>AEYVRALFDFNGNDEEDLP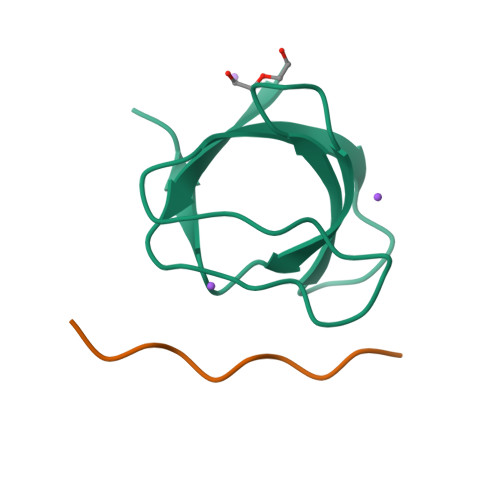FKKGDILRIRDKPEEQWWNAEDSEGKRGMIPVPYVEKYR[2x];>XYEKPALPRKRX[2x]> GSHMIQAYLGLGSNIGDRESQLNDAIKILNEYDGISVSNISPIYETAPVGYTEQPNFLNLCVEIQT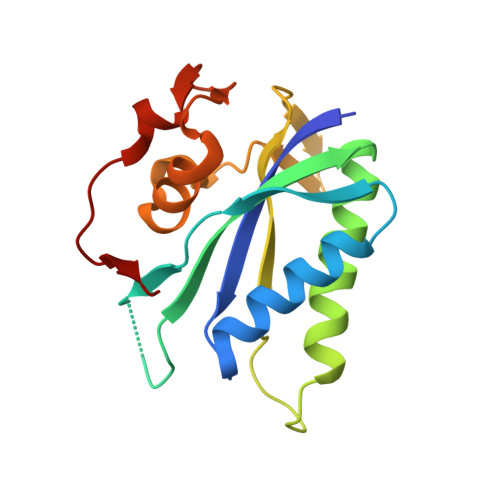TLTVLQLLECCLKTEECLHRIRKERWGPRTLDVDILLYGEEMIDLPKLSVPHPRMNERAFVLIPLNDIAANVVEPRSKLKVKDLVFVDDSVKRYK>[3x]VRIRRAGLEDLPGVARVLVDTWRATYRGVVPEAFLEG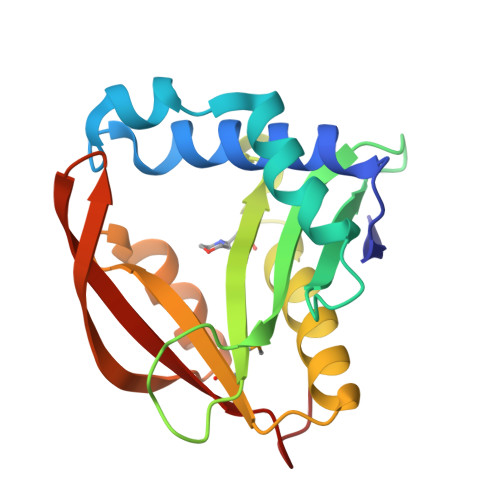LSYEGQAERWAQRLKTPTWPGRLFVAESESGEVVGFAAFGPDRASGFPGYTAELWAIYVLPTWQRKGLGRALFHEGARLLQAEGYGRMLVWVLKENPKGRGFYEHLGGVLLGEREIELGGAKLWEVAYGFDLGGHKW> QAQITGRPEWIWLALGTALMGLGTLYFLVKGMGVSDPDAKKFYAITTLVPAIAFTMYLSMLLGY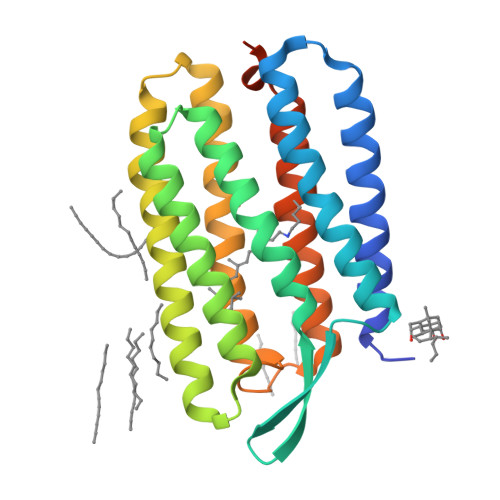GLTMVPFGGEQNPIYWARYADWLFTTPLLLLDLALLVDADQGTILALVGADGIMIGTGLVGALTKVYSYRFVWWAISTAAMLYILYVAFFGFTSKAESMRPEVASTFKVLRNVTVVLWSAYPVVWLIGSEGAGIVPLNIETLLFMVLDVSAKVGFGLILLRSRAIFGEAEAPEPSAGDGAAATSD> GAASMRQNPPKEPSEEEVLQYIVDNVNKLLSRHYSLVEFDAIQGTDLLQILADIFGTLSPAQQIDMGVAPTDEAAASMLEFLTKTLGYRVPPMLADSFPTSFSRAEPTVIYPTLYWVLSNMQQNEKRVYLARFLQRLEIPEAMLAQDEDVRALYQQYVNLRGMFVNTHRRVDALRTAHADPADARRAVTVLEEECDRLRGYIQVAEKKLAGVPDKEALLNACKSLRAALEEESRLAEKGVELQQQLISSRQRSTEMHNRLQNLRRDAADGRVDVIVRRLRDEIQTNKMIIEEQLPKELQQKQRENAEFDRLISEPLDMQALTTENQQLDEALKKLHQQVKERQKPGED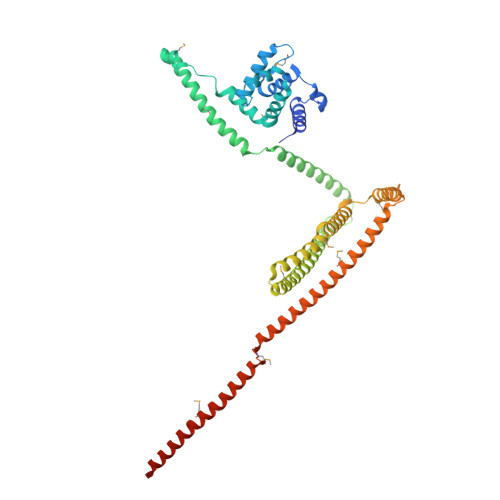GSTIATIKQQVERVAKRKVEVMEQLTGLQADNSRTLNDIRERENRIEQLREAHHMLKDDDFREFSKQVLAKKAATESMRTHLSEQRVEYGVLNFTENVLRSQFTSL> MIKVEIKPSQAQFTTR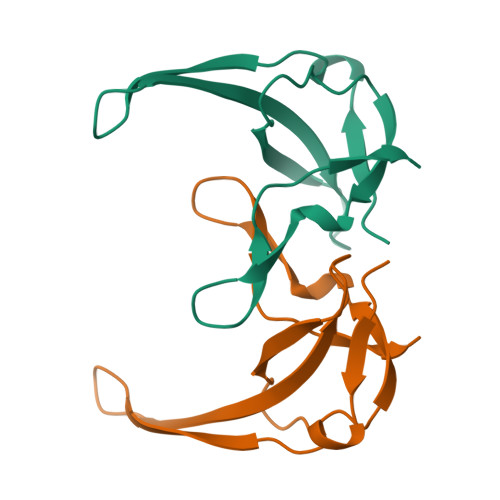SGVSRQGKPYSLNEQLCYIDLGNEYPVLVKMTLDEGQPAYAPGLYTVHLSSFKVGQFGSLMIDRLRLVPAK The BisI family of restriction endonucleases is unique in requiring multiple methylated or hydroxymethylated cytosine residues within a short recognition sequence (GCNGC), and in cleaving directly within this sequence, rather than at a distance. We present the crystal structures of NhoI and Eco15I_Ntd (N-terminal catalytic domain of Eco15I) in the absence of DNA and in specific complexes with fully methylated GCNGC containing dsDNA. Both proteins are homodimeric, with each domain involved in target sequence recognition and catalysis. The crystal structures show that the modified cytosine bases are recognized in the context of double-stranded DNA, without base flipping.

As the crystals of the specific NhoI DNA complex diffracted far better than other crystals, the following structural description focuses largely on this complex. The DNA in the NhoI–DNA complex is bound in both orientations that are compatible with the 2-fold symmetry of the enzyme. This does not compromise the electron density for the base pairs that follow the two-fold symmetry, i.e. of the external and internal G:5mC pairs. However, it somewhat blurs the density for the central symmetry breaking base pair, and for the flanking base pairs that do not follow the 2-fold symmetry. The external 5mC, and the paired guanine, do not form a single direct hydrogen bond with the protein. Instead, there are only water mediated hydrogen bonds from the proximal subunit on the major groove side (Thr144, Ser137), and from the distal subunit to the minor groove side (Asn42, Ser65). Recognition of the internal 5mC is more stringent, with a purine selecting hydrogen bond from the Ser98 (partially conserved) to the N7 of the paired guanine, and a G:C or G:5mC pair selecting hydrogen bond in the central minor groove from the guanine to Asn42. In NhoI, the pocket for an external methyl group (GCNG5mC) is formed by the proximal enzyme subunit, namely by the Cβ of Ser98 and the side chain of Arg84, with the side chain of Gln96 only slightly further apart. For both NhoI and Eco15I, these are a histidine and a valine of the distal subunit (His139 and Val140 in NhoI). In NhoI, a guanidino group of an arginine residue nearby (Arg101 of the proximal NhoI subunit) also contributes to the internal methyl binding pocket.

>[5x]GSMSRPPSYAGDMNLENLTTRELLAVSRASLRELKRRGVIRSGNAPAGDYAELLVQRATDGELANASQKSWDIRTTEGDRLQVKARVITDEHANGERQLSTIRSWDFDAAVIVLFDDNFRVWRAARVPAAIMKEAAYYSQHVRGYTVYAKDALLNHSEVEDWTEQLRSVEQ>[2x]SEKSEEINEKDLRKKSELQGTALGNLKQIYYYNEKAKTENKESHDQFLQHTILFKGFFTDHSWYNDLLVDFDSKDIVDKYKGKKVDLYGAYYGYQCAG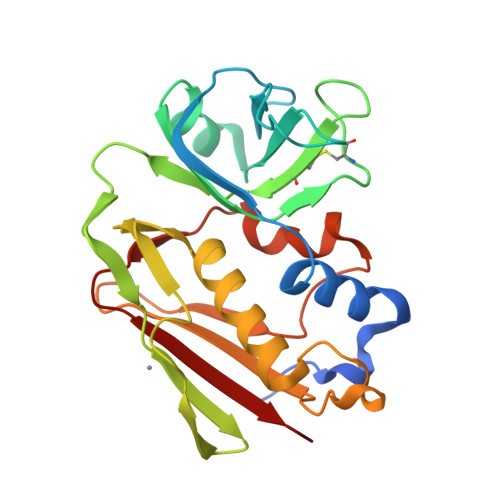GTPNKTACMYGGVTLHDNNRLTEEKKVPINLWLDGKQNTVPLETVKTNKKNVTVQELDLQARRYLQEKYNLYNSDVFDGKVQRGLIVFATSTEPSVNYDLFGAQGQYSNTLLRIYRDNKTINSENMHIDIYLYTS> MPLELTQSRVQKIWVPVDHRPSLPRSCGPKLTNSPTVIVMVGLPARGKTYISKKLTRYLNWIGVPTKVFNVGEYRREAVKQYSSYNFFRPDNEEAMKVRKQCALAALRDVKSYLAKEGGQIAVFDATNTTRERRHMILHFAKENDFKAFFIESVCDDPTVVASNIMEVKISSPDYKDCNSAEAMDDFMKRISCYEASYQPL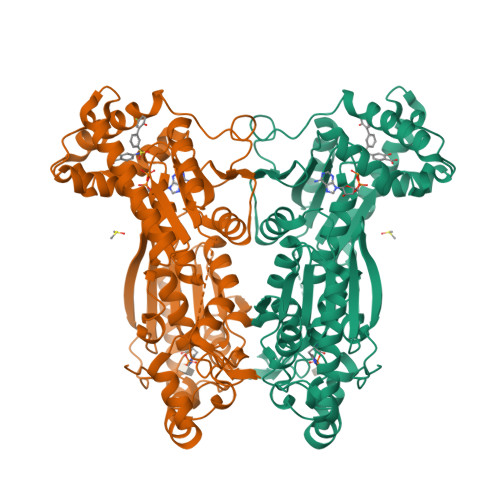DPDKCDRDLSLIKVIDVGRRFLVNRVQDHIQSRIVYYLMNIHVQPRTIYLCRHGENEHNLQGRIGGDSGLSSRGKKFASALSKFVEEQNLKDLRVWTSQLKSTIQTAEALRLPYEQWKALNEIDAGVCEELTYEEIRDTYPEEYALREQDKYYYRYPTGESYQDLVQRLEPVIMELERQENVLVICHQAVLRCLLAYFLDKSAEEMPYLKCPLHTVLKLTPVAYGCRVESIYLNVESVCTHRERSEDAKKGPNPLMRRNSVTPLASPEPTKKPRINSFEEHVASTSAALPSCLPPEVPTQLPGQNMKGSRSSADSSRKH> SNCSRDTGDELMAALLAEGINLILPPRDNIAPGDLIIADPQGGARLGGWHEVFNLQLSPEVATDPGFKSFQFRASSILQVGVAASVMGRVLQALGLGSGSFSSAFSSSNADTIQLSIVAPANKELTN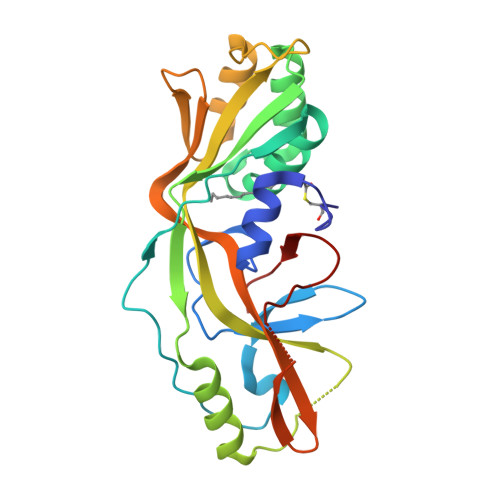FDAVLVQMNEAKAEPAQGYTDRNFFVVTKVWRARGIRISVADKSKKQVDLSAKAVEELTAKAKMELKREDTGSYAFLAASQLIFGLTLREVTYKDGAIVDVAPTGPLKFRGKGPGDPFAFIGDDAFVDLPES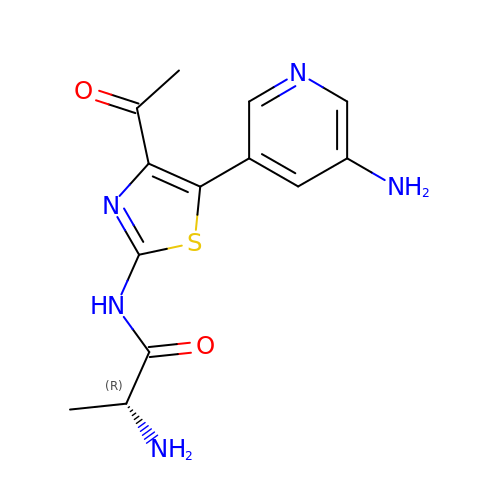(2~{R})-2-azanyl-~{N}-[5-(5-azanylpyridin-3-yl)-4-ethanoyl-1,3-thiazol-2-yl]propanamide | C13 H15 N5 O2 S | DVUMUHRRODTQIU-ZCFIWIBFSA-N1-hydroxydodecan-4-one | 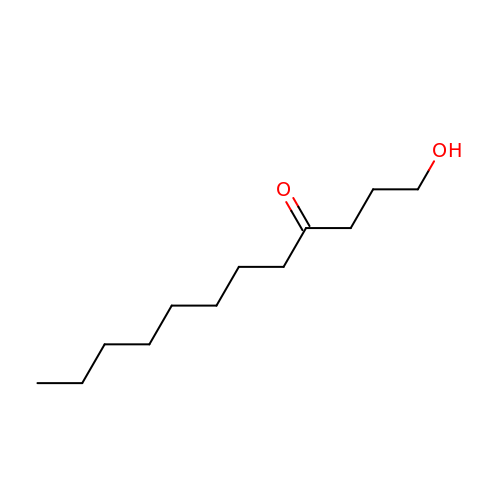C12 H24 O2 | ZWRNUBJKJQOMRO-UHFFFAOYSA-N> MCPQKLTISWFAIVLLVSPLMAMWELEKDVYVVEVDWTPDAPGETVNLTCDTPEEDDITWTSDQRHGVIGSGKTLTITVKEFLDAGQYTCHKGGETLSHSHLLLHKKENGIWSTEILKNFKNKTFLKCEAPNYSGRFTCSWLVQRNMDLKFNIKSSSSSPDSRAVTCGMASLSAEKVTLDQRDYEKYSVSCQEDVTCPTAEETLPIELALEARQQNKYENYSTSFFIRDIIKPDPPKNLQMKPLKNSQVEVSWEYPDSWSTPHSYFSLKFFVRIQRKKEKMKETEEGCNQKGAFLVEKTSTEVQCKGGNVCVQAQDRYYNSSCSKWACVPCRVRSGTKHHHHHH

Here, we present the use of the GlycoDelete (GD) HEK cell line for protein crystallization, which produces homogeneous mature-like trisaccharide glycan stubs. The GD cell line is derived from the HEK293S MGAT1−/− cell line and has been transformed with Golgi-resident EndoT (an endo-β-N-acetyl­glucosaminidase similar to EndoH). This enzyme processes the Man5GlcNAc2 glycans, allowing the NG to be further processed by native Golgi-resident enzymes to generate mature-like glycans consisting of one GlcNac (which can be fucosylated), one galactose (Gal) and one sialic acid (Neu5Ac). The glycan stubs do not need further enzymatic processing, and we show that for heavily glycosylated fragments of human colony-stimulating factor 1 receptor (CSF-1R), murine IL-12B and human Down syndrome cell-adhesion molecule (DSCAM) the NG modifications facilitate the production of diffraction-quality crystals.

IL-12B is a soluble cytokine receptor-like protein associated with the heterodimeric pro-inflammatory cytokines interleukin-12 (IL-12) and interleukin-23 (IL-23). IL-12B is secreted as a monomer (denoted IL-12p40) and as a homodimer (denoted IL-12p80). IL12B can also form a disulfide-linked interaction mediated by Cys197 on murine IL-12p40 to form heterodimeric cytokines with the IL-12p35 subunit, resulting in IL-12, or the IL-23p19 subunit, resulting in IL-23. The crystallographic twofold axis present in the I41 lattice is located at Cys197, thereby forming a crystallographic homodimer. Aside from the homotypical disulfide, the interface area is very limited in size (287 Å2) and lacks specific interactions (13 interface residues per protomer and no hydrogen bonds or salt bridges). The electron density allows the modeling of a Man4GlcNAc2 glycan. The immature glycan is located between the D1 and D2 domains and may be difficult to access by the EndoT enzyme. Although the GD cell line was engineered to alter the glycosylation machinery, it does not affect the formation and retention of the immature glycan. We conclude that it is a critical feature of the GD cell line that the glycosylation is only reduced after it passes into the Golgi, as it retains the capability to secrete glycoproteins that require immature glycans for folding. The immature glycan was clearly present in the crystal structure of IL-12B based on recombinant protein produced by GD cells, illustrating the general versatility of this cell line for structural biology applications.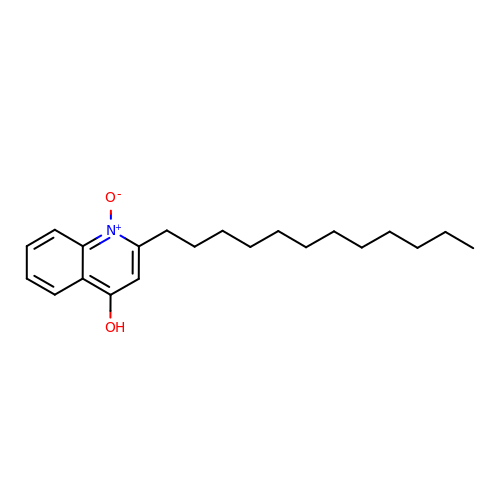2-dodecyl-1-oxidanidyl-quinolin-1-ium-4-ol | C21 H31 N O2 | DAHXHNYLVGWOJA-UHFFFAOYSA-N> MSGIALSRLAQERKAWRKDHPFGFVAVP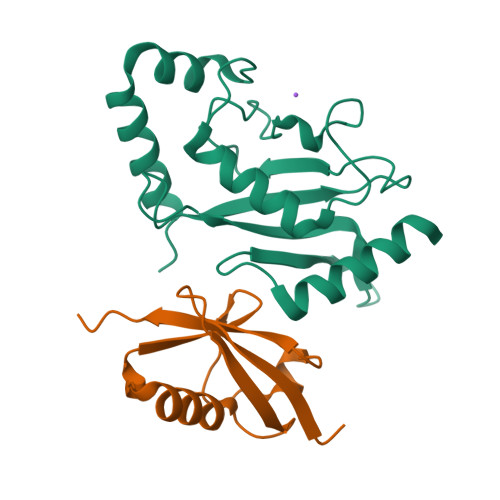TKNPDGTMNLMNWECAIPGKKGTPWEGGLFKLRMLFKDDYPSSPPKCKFEPPLFHPNVYPSGTVSLSILEEDKDWRPAITIKQILLGIQELLNEPNIQDPAQAEAYTIYCQNRVEYEKRVRAQAKKFAPS;> MEYIKLKVIGQDSSEIHFKVKMTTHLKKLKESYCQRQGVPMNSLRFLFEGQRIADNHTPKELGMEEEDVIEVYQEQTGG>[9x]MPVIKPVIVAVSSAPVSTGGVIATTVSPTVAR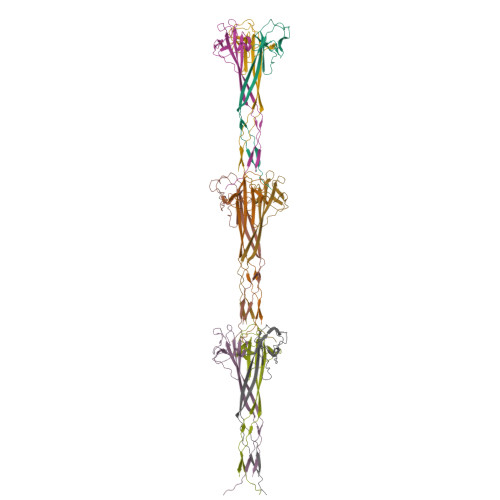FYAAITAAMIAGGVTTIPAASFLDDADAPVAALPVPAANGYYNVYINGILQQGGLSTLTAVSLALASGDFVEGTPVLLEVGTFGGDSTLTTQPTISAPTITIIS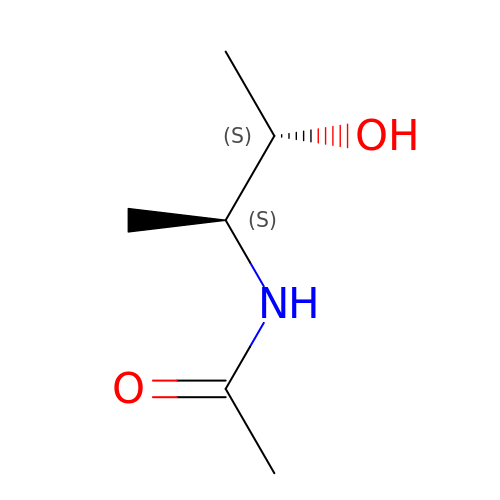~{N}-[(2~{S},3~{S})-3-oxidanylbutan-2-yl]ethanamide | C6 H13 N O2 | ZCGNIFXXTKDQRT-WHFBIAKZSA-N> MEHVAFGSEDIENTLAKMDDGQLDGLAFGAIQLDGDGNILQXNAAEGDITGRDPKQVIGKNFFKDVA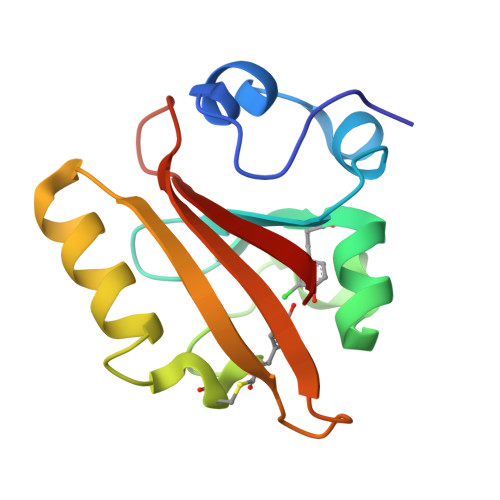PCTDSPEFYGKFKEGVASGNLNTMFEYTFDYQMTPTKVKVHMKKALSGDSYWVFVKRV> LKELIASNPDDLTTELKRAFRPLTPHIAIDGNELDALTILVNLTDKTDDQKDLLDRAKCKQKLRDEKWWASCINCVNYRQSHNPKFPDIRSEGVIRTQALGELPSFLLSSSKIPPYHWSYSHDSKYVNKSAFLTNEFCWDGEISCLGELLKDADHPLWNTLKKLGCSQKTCKAMAKQLADITLTTINVTLAPNYLTQISLPDSDTSYISLSPVASLSMQSHFHQRLQDENRHSAITRFSRTTNMGVTAMTCGGAFRMLKSGAKFSSPPHHRLNNGSFLVLPNIRVCGATAL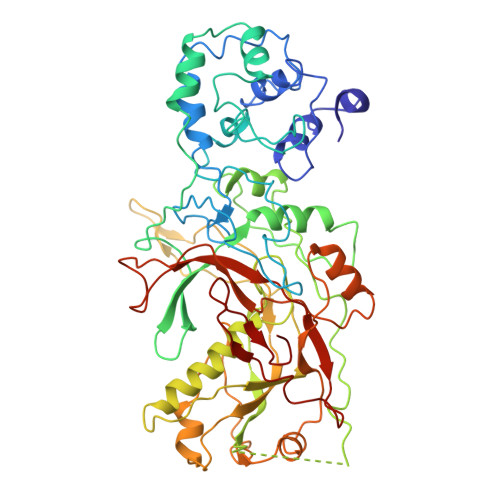SSPVTVGIPSLTAFFGFVHAFERNINRTTSSFRVESFAICVHQLHVEKRGLTAEFVEKGDGTISAPATRDDWQCDVVFSLILNTNFAQHIDQDTLVTSLPKRLARGSAKIAIDDFKHINSFSTLETAIESLPIEAGRWLSLYAQSNNNLSDLLAAMTEDHQLMASCVGYHLLEEPKDKPNSLRGYKHAIAECIIGLINSITFSSETDPNTIFWSLKNYQNYLVVQPRSIN>[2x]MVLYFIGLGLYDERDITVKGLEIAKKCDYVFAEFYTSLMAGTTLGRIQKLIGKEIRVLSREDVELNFENIVLPLAKENDVAFLTPGDPLVATTHAELRIRAKRAGVESYVIHAPSIYSAVGITGLHIYKFGKSATVAYPEGNWFPTSYYDVIKENAERGLHTLLFLDIKAEKRMYMTANEAMELLLKVEDMKKGGVFTDDTLVVVLARAGSL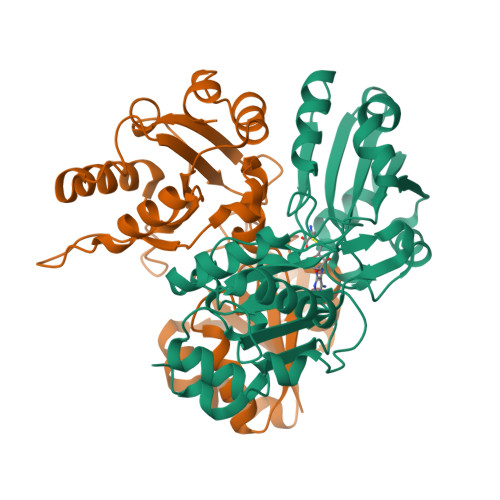NPTIRAGYVKDLIREDFGDPPHILIVPGKLHIVEAEYLVEIAGAPMEILRVNV> QFAKPEDAVKYRQSALTLMASHFGRMTPVVKGQAPYDAAQIKANVEVL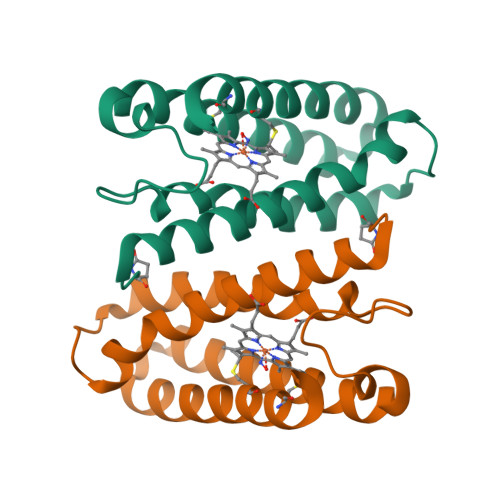KTLSALPWAAFGPGTEGGDARPEIWSDAASFKQKQQAFQDNIVKLSAAADAGDLDKLRAAFGDVGASCKACHAAYRKKK> KRYS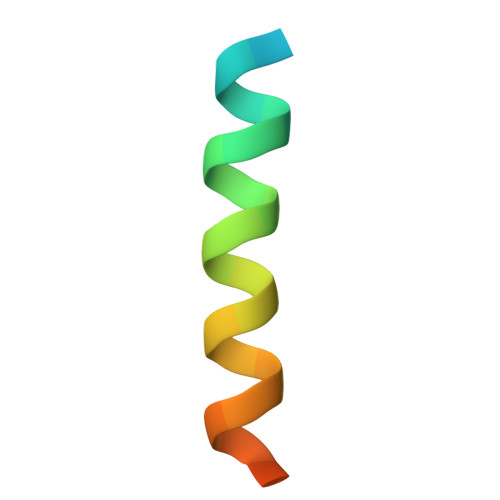ALSNDISQGIKRQRMTVESMGWALS>[2x]SAAVESFVTKQLDLLELERDAEVEERRSWQENISLKELQSRGVCLLKLQVSSQRTGLYGRLLVTFEPRRYGSAAALPSNSFTSGDIVGLYDAANEGSQLATGILTRVTQKSVTVAFDESHDFQQSLDRENSYRLLKLANDVTYRRLKKALIALKKYHSGPASSLIEVLFGRSAPSPASEIHPLTFFNTCLDTSQKEAVLFALSQKELAIIHGPPGTGKTTTVVEIILQAVKQGLKVLCCAPSNIAVDNLVERLALCKQRILRLGHPARLLESIQQHSLDAVLARSDSAQ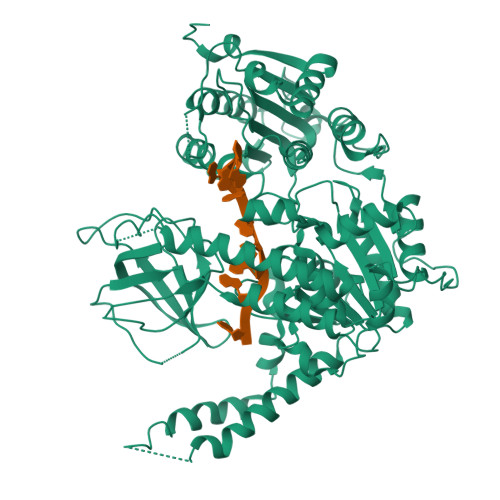IVADIRKDIDQVFVKNKKTQDKREKSNFRNEIKLLRKELKEREEAAMLESLTSANVVLATNTGASADGPLKLLPESYFDVVVIDECAQALEASCWIPLLKARKCILAGDHKQLPPTTVSHKAALAGLSLSLMERLAEEYGARVVRTLTVQYRMHQAIMRWASDTMYLGQLTAHSSVARHLLRDLPGVAATEETGVPLLLVDTAGCGLFELEEEDEQSKGNPGEVRLVSLHIQALVDAGVPARDIAVVSPYNLQVDLLRQSLVHRHPELEIKSVDGFQGREKEAVILSFVRSNRKGEVGFLAEDRRINVAVTRARRHVAVICDSRTVNNHAFLKTLVEYFTQHGEVRTAFEYLDDIVP(2E,5S)-5-methylhept-2-enoic acid | C8 H14 O2 | 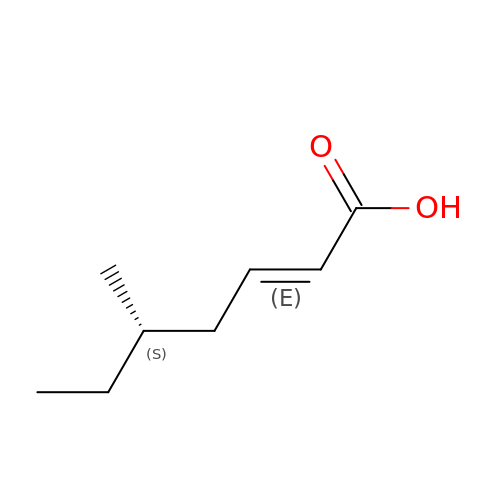WCNAROBWFNTKGN-KNIZRNDPSA-N>[2x]GPMLADLDHFGKNYKHDEEAQRNQKPWMLTWPQIKLVLLAGVGFFLDAYDLFIINQVAPMLAQVYFPKTGLPAQRQDLMKAAANIGCVVGQVMFGVLGDSFGRKFVYGKELILIIVATIFQMSAPSHWDGNRVLTWITICRVFLGIGIGGDYPMSATVVSDRANIHRRGTLLCFIFANQGWGSFVGSLVTIVTISGFKHRLKSGHTHDVDKAWRILIGLSLIPAFGTLYQRLTLPESRKFELTRDAASSSTVAIDKKDHDATHEVKDAPESEKSSPKVTPADAIDDDRHGVIASKKAHWQEFVAYFSTWNHFRNLLGSMLGWFLVDIAFYGIN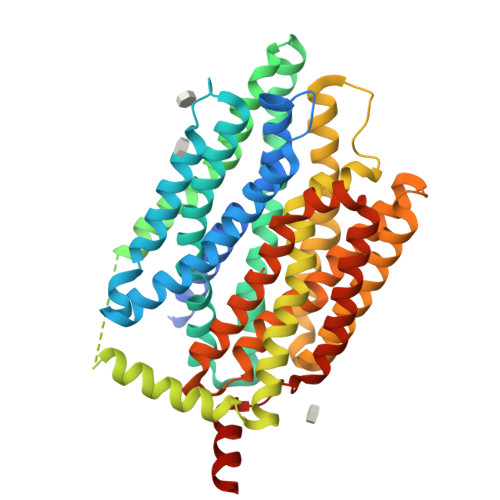LNQSVVLAQIGFAGKTGDVYDKLFQLATGNIIVTALGFLPGYYFTLFLIDIVGRKKLQFMGFIMSGLFLAILAGEIDHIGKGPLLACFTFMQFFFNFGANTTTFIVAAELFPTRIRASAHGISAAAGKCGAILSSLVFNQLKAKIGTSAVLWIFFSTCILGFISTFLIDETMGVDPDEKDLEERRARGEIPGGLVPR> GAGCAGACCTGACGACAAT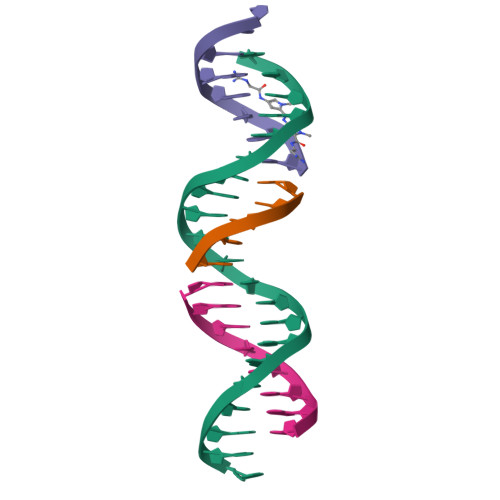TA;> TCGTC;> TCTAATTG;> AGGTCTGC2-(difluoromethoxy)benzene-1-sulfonamide 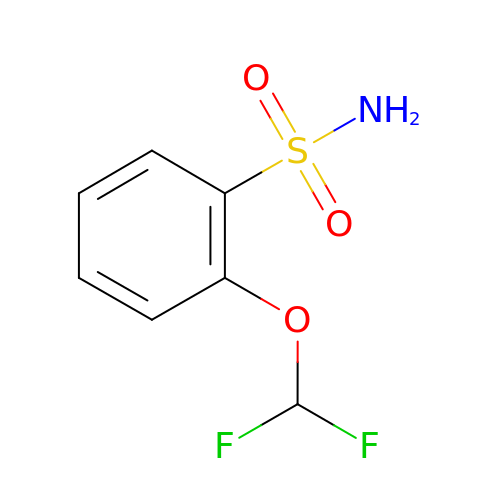| C7 H7 F2 N O3 S | XDODAVQVIOWLPT-UHFFFAOYSA-N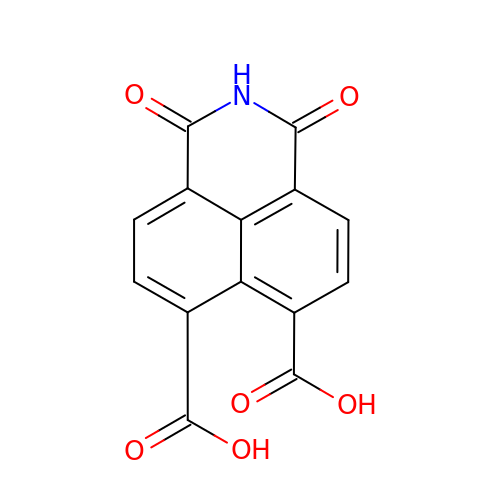1,3-bis(oxidanylidene)benzo[de]isoquinoline-6,7-dicarboxylic acid | C14 H7 N O6 | NFOKRVXFAWSKMU-UHFFFAOYSA-N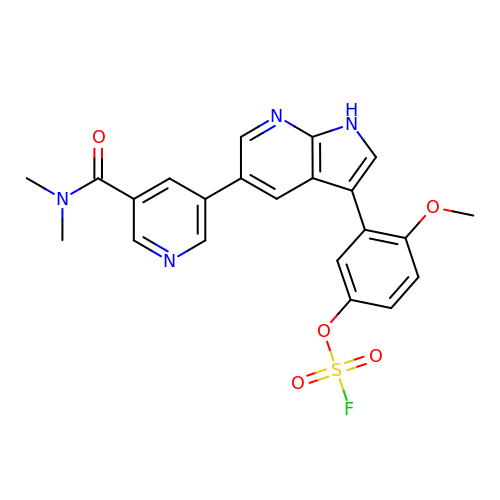5-[5-(dimethylcarbamoyl)pyridin-3-yl]-3-(5-fluorosulfonyloxy-2-methoxy-phenyl)-1H-pyrrolo[2,3-b]pyridine | C22 H19 F N4 O5 S | NPCQFNRTXVLCCU-UHFFFAOYSA-N> ASNLKIVRMDRTAGCVTGGEEIMLLCDKVQKDDIQIRFYEEEENGGVWEGFGDFSPTDVHRQFAIVFKTPKYKDVNITKPASVFVQLRRKSD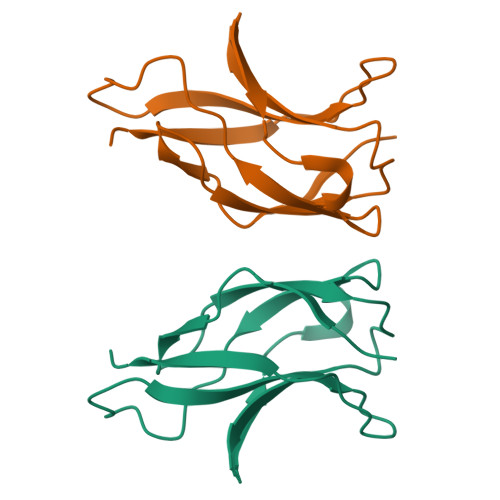LETSEPKPFLYYPE>[2x]MSNLKDFSQPGSGQESNFGVDFVIHYKVPAAERDEAEAGFVQLIRALTTVGLATEVRHGENESLLVFVKVASPDLFAKQVYRARLGDWLHGVRVSAPHNDIAQALQDEPVVEAERLRLIYLMITKPHNEGGAGVTPTNAKWKHVESIFPLHSHSFNKEWIKKWSSKYTLEQTDIDNIRDKFGESVAFYFAFLRSYFRFLVIPSAFGFGAWLLLGQFSYLYALLCGLWSVVFFEYWKKQEVDLAVQWGVRGVSSIQQSRPEFEWEHEAEDPITGEPVKVYPPMKRVKTQLLQIPFALACVVAAGALIVTCNSLEVFINEVYSGPGKQYLGFLPTIFLVIGTPTISGVLMGAAEKLNAMENYATVDAHDAALIQKQFVLNFMTSYMALFFTAFVYIPFGHILHPFLNFWRATAQTLTFSEKELPTREFQINPARISNQMFYFTVTAQIVNFATEVVVPYIKQQAFQKAKQLKSGSKVQEDHEEEAEFLQRVREECTLEEYDVSGDYREMVMQFGYVAMFSVAWPLAACCFLVNNWVELRSDALKIAISSRRPIPWRTDSIGPWLTALSFLSWLGSITSSAIVYLCSNSKNGTQGEASPLKAWGLLLSILFAEHFYLVVQLAVRFVLSKLDSPGLQKERKERFQTKKRLLQENLGQDAAEEAAAPGIEHSEKITREALEEEARQASIRGHGTPEEMFWQRQRGMQETIEIGRRMIEQQLAAGKNGKKSAPAVPSEKAS

The breakthrough X-ray structure of a fungal TMEM16 homologue, nhTMEM167, revealed that TMEM16 proteins are homo-dimers. Each subunit is composed of 10 transmembrane (TM) segments, with structured termini on the cytoplasmic side and featuring a polar cavity (groove) that faces the lipid membrane and serves as the permeation pathway. TM6 and TM7 also participate in the formation of the two regulatory Ca2+ binding sites located within the membrane. Our results illuminate the detailed molecular mechanism by which the lipid groove of the nhTMEM16 scramblase can rearrange from a membrane-exposed conformation to an intermediate state that is occluded from the membrane, forming an ion-conductive conformation.

Hydrophobic interactions between TM4 and TM3 that keep the groove open are strengthened by I343 and L347 in TM4, and L302 in TM3. To relate the mechanistic hypothesis to structural determinants, we used single particle cryo-EM to determine the structure of the L302A mutant reconstituted in lipid nanodiscs in the presence of 0.5 mM Ca2+, to a resolution of 4.0 Å. The predicted disruption of the interaction between TM3 and TM4 is validated by the observed increases in distance between A302 on TM3 and I343/L347 on TM4 from 3.7 to 7.4 Å and from 5.0 to 7.2 Å. This causes the repositioning of TM3, which slides upwards and away from TM5 and TM6, and of TM4, which tilts away from TM3 and TM5 and toward TM6, bringing T333 and V337 of TM4 to interact with Y439, T443, and V447 from TM6. With a minimum inner diameter > 2.9 Å, this pore is compatible with the movement of permeant monovalent cations such as Na+ or K+ while sterically precluding passage of large cations, such as NMDG+, which are not conducted by nhTMEM1624. Thus, the L302A mutant loses most of its lipid scrambling activity while maintaining significant channel function.>XGELAAIKQELAAIKKELAAIKYELAAIKQGX[3x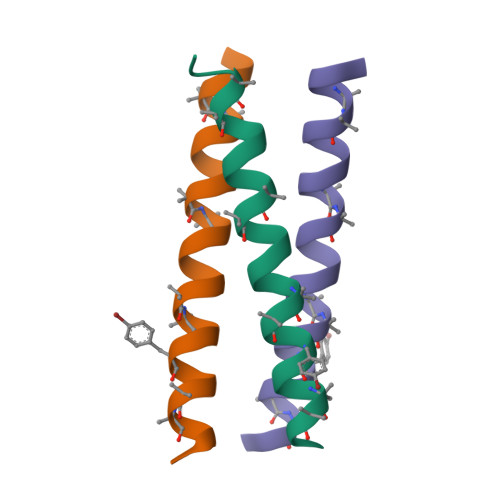]>[2x]MEDPRRRTTAPRAKKPSAKRAPTQPSRTRAHAESCGPQRGARSRRAERDGDTTEKPRAPGPRVHPARATELTKDAQPSAMDAAGATARPAVRVPQQQAILDPELPAVREPQPPADPEARKVVRGPSHRRGARSTGQPRAPRGSRKEPDKLKKVLDKLRLKRKDISEAAETVNKVVERLLRRMQKRESEFKGVEQLNTGSYYEHVKISAPNEFDVMFKLEVPRIELQEYYETGAFYLVKFKRIPRGNPLSHFLEGEVLSATKMLSKFRKIIKEEVKEIKDIDVSVEKEKPGSPAVTLLIRNPEEISVDIILALESKGSWPISTKEGLPIQGWLGTKVRTNLRREPFYLVPKNAKDGNSFQGETWRLSFSHTEKYILNNHGIEKTCCESSGAKCCRKECLKL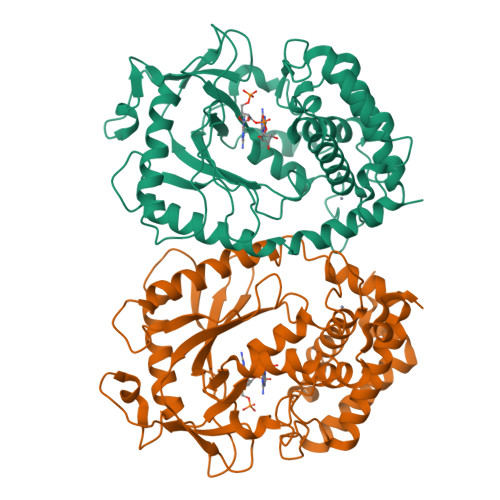MKYLLEQLKKEFQELDAFCSYHVKTAIFHMWTQDPQDSQWDPRNLSSCFDKLLAFFLECLRTEKLDHYFIPKFNLFSQELIDRKSKEFLSKKIEYERNNGFPIFDKL> GSESDSGMASQADQKEEELLLFWTYIQAMLTNLESLSLDRIYNMLRMFVVTGPALAEIDLQELQGYLQKKVRDQQLVYSAGVYRLPKNCS;> GSARGPVGKRLQQELMTLMMSGDKGISAFPESDNLFKWVGTIHGAAGTVYEDLRYKL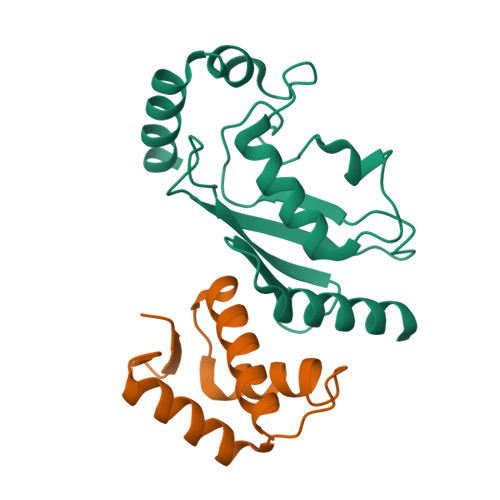SLEFPSGYPYNAPTVKFLTPCYHPNVDTQGNICLDILKEKWSALYDVRTILLSIQSLLGEPNIDSPLNTHAAELWKNPTAFKKYLQETYSKQVTSQEP>[2x]MTTVIDATMAYRFLEEATDSSSSSSSSKLESSPVDAVLFVGMSLVLGIASRHLLRGTRVPYTVALLVIGIALGSLEYGAKHNLGKIGHGIRIWNEIDPELLLAVFLPALLFESSFSMEVHQIKRCLGQMVLLAVPGVLISTACLGSLVKVTFPYEWDWKTSLLLGGLLSATDPVAVVALLKELGASKKLSTIIEGESLMNDGTAIVVFQLF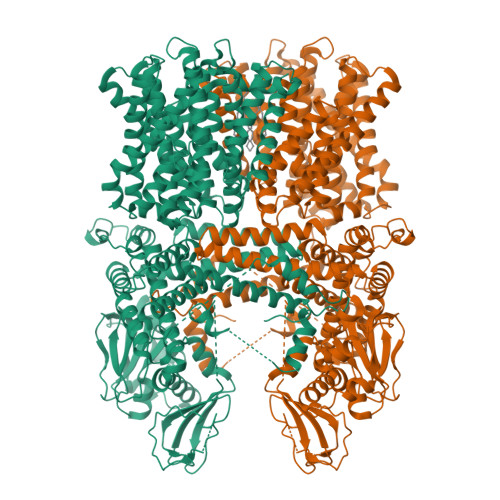LKMAMGQNSDWSSIIKFLLKVALGAVGIGLAFGIASVIWLKFIFNDTVIEITLTIAVSYFAYYTAQEWAGASGVLTVMTLGMFYAAFARTAFKGDSQKSLHHFWEMVAYIANTLIFILSGVVIAEGILDSDKIAYQGNSWRFLFLLYVYIQLSRVVVVGVLYPLLCRFGYGLDWKESIILVWSGLRGAVALALSLSVKQSSGNSHISKETGTLFLFFTGGIVFLTLIVNGSTTQFVLRLLRMDILPAPKKRILEYTKYEMLNKALRAFQDLGDDEELGPADWPTVESYISSLKGSEGELVHHPHNGSKIGSLDPKSLKDIRMRFLNGVQATYWEMLDEGRISEVTANILMQSVDEALDQVSTTLCDWRGLKPHVNFPNYYNFLHSKVVPRKLVTYFAVERLESACYISAAFLRAHTIARQQLYDFLGESNIGSIVINESEKEGEEAKKFLEKVRSSFPQVLRVVKTKQVTYSVLNHLLGYIENLEKVGLLEEKEIAHLHDAVQTGLKKLLRNPPIVKLPKLSDMITSHPLSVALPPAFCEPLKHSKKEPMKLRGVTLYKEGSKPTGVWLIFDGIVKWKSKILSNNHSLHPTFSHGSTLGLYEVLTGKPYLCDLITDSMVLCFFIDSEKILSLQSDSTIDDFLWQESALVLLKLLRPQIFESVAMQELRALVSTESSKLTTYVTGESIEIDCNSIGLLLEGFVKPVGIKEELISSPAALSPSNGNQSFHNSSEASGIMRVSFSQQATQYIVETRARAIIFNIGAFGADRTLHRRPSSLTPPRSSSSDQLQRSFRKEHRGLMSWPENIYAKQQQEINKTTLSLSERAMQLSIFGSMVNVYRRSVSFGGIYNNKLQDNLLYKKLPLNPAQGLVSAKSESSIVTKKQLETRKHACQLPLKGESSTRQNTMVESSDEEDEDEGIVVRIDSPSKIVFRNDL> MAATSSSDSDGGKGESEANSKWLDSLSDSMANIHTFSACLALADFHGDGEYKLAMGDLGPDGRQPRLKVLKGHTLVSQKPLPDLPAAAVTFLMASHEPRTPALAIASGPCVYVYKNLKPYFKFSLPSLPTNPLEQDLWNQAKEDQIDPLTLKEMLEGIREKAEVPLSVQSLRFLPLELSEMEAFVNQHKSKSIRRQTVITTMTTLKKNLADEDAVSCLVLGTENKELLVLDPEAFTILAKMSLPSVPAFLEASGQFDVEFRLAAACRNGSIYILRRDSKRPKYCIELGAQPVGLVGVHKVLVVGSNQDSLHGFTYKGKRLWTVQMPAAILAMNLLEQHSRGLQAVMAALANEEVRIYHDKVLLNVIRTPEAVTSLCFGRYGREDNTLIMTTLGGGLIIKILKRTAVFAEGGGEAGPPPSQAIKLNV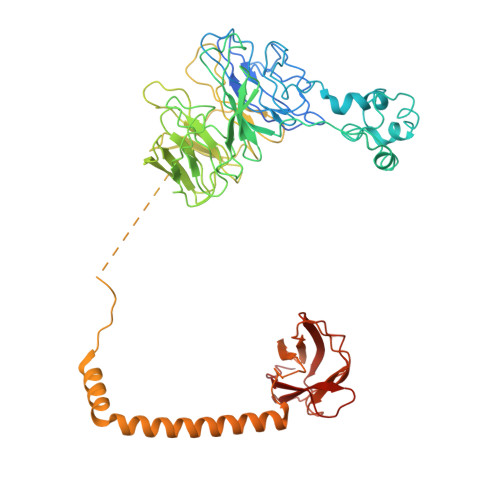PRKTRLYVDQTLREREAGTAMHRTFQADLYLLRLRAARAYVQALESSLSPVSLTAREPLKLHAVVQGLGPTFKLTLHLQNTSTARPILGLVVCFLYNEVLYALPRAFFKVPLLVPGLNYPLETFVKSLSDKGISDIIKVLVLREGQSTPLLSAHINMPMSEGLAAD Neuroglobin (Ngb) is a phylogenetically ancient representative of the globin superfamily found in vertebrates and predominantly expressed in the central nervous system at overall concentrations lower than 1 μM, thus excluding a role in dioxygen storage or transport. At difference with Mb, in the absence of exogenous ligands, Ngb is endowed with heme iron hexacoordination by two conserved histidines: the distal His64 and the proximal His96.8−11 This peculiarity of Ngb induces a complex binding kinetics and conformational rearrangement upon ligation. Ligand binding to the ferrous heme of Ngb is limited by the rate of rupture of the iron–His64 bond, allowing diatomic gases to compete for the vacant sixth coordination position. Notably, the dissociation of His64 and the subsequent diatomic gas (O2, NO, CO) ligation to the ferrous iron triggers the sliding of the heme deeper inside the internal Ngb hydrophobic cavity and the movement of loops such as the CDloop and the EFloop. Moreover, molecular dynamics predictions suggested that Ngb residues, in particular, those forming the CDloop–D-helix segment, interact with cytochrome c and Gα(i) proteins, underlying the molecular basis of Ngb signaling role.

We produced a neuroglobin variant, namely, Ngb CDless, with the excised CDloop- and D-helix, directly joining the C- and E-helices. We determined the crystal structure of the ferric murine Ngb CDless mutant at a 1.8 Å resolution, which according to Arcovito et al. is structurally indistinguishable from the reduced ferrous structure. The analysis of the crystallographic data yielded the observation of two murine Ngb mutant conformational substates (MON1 and MON2) in the same crystal. Consistently, the refinement of the heme density for Ngb CDless MON1 and MON2 indicated the presence of a double heme insertion, along with double conformations for His64 and His96, in proportions similar to those previously reported. More in detail, the refinement based on the residual Fc–Fo difference map allowed us to estimate that canonical and reversed hemes are present in a 29:71 and 33:67 ratio in MON1 and MON2, respectively. Iterative rounds of modeling and refinement enabled us to reconstruct the protein segment between the C- and E-helices (CElink) of MON1. However, the poorly defined electronic density for this region in MON2 prevented the determination of the CElink structure between Phe42 and Pro59, suggesting a highly mobile conformation. Analysis of the structure showed that the lack of D-helix and of Phe49 in Ngb CDless triggers the flipping of Phe61 to the surface of MON2, followed by Phe28 to maintain π–π stacking, causing a displacement of the Phe32 side chain toward the bulk. Conversely, MON1, with a defined position of the CElink, appears to preserve the arrangement of the hydrophobic core, retaining the heme crevice observed in Ngb wild type.

>[2x]HMERPESELIRQSWRVVSRSPLEHGTVLFARLFALEPSLLPLFGSSPEFLDHIRKVMLVIDAAVTNVEDLSSLEEYLTSLGRKHRAVGVRLSSFSTVGESLLYMLEKSLGPDFTPATRTAWSRLYGAVVQAMSRGWDGE> FKSVSYWGFGR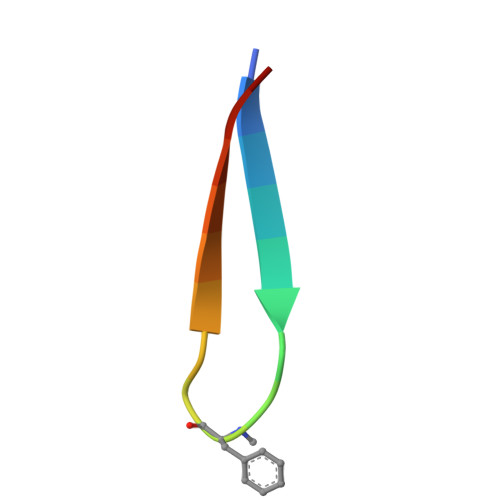LSYYNHC>[2x]MNLKALPAIEGDHNLKNYEETYRHFDWAEAEKHFSWHETGKLNAAYEAIDRHAESFRKNKVALYYKDAKRDEKYTFKEMKEESNRAGNVLRRYGNVEKGDRVFIFMPRSPELYFIMLGAIKIGAIAGPLFEAFMEGAVKDRLENSEAKVVVTTPELLERIPVDKLPHLQHVFVVGGEAESGTNIINYDEAAKQESTRLDIEWMDKKDGFLLHYTSGSTGTPKGVLHVHEAMIQQYQTGKWVLDLKEEDIYWCTADPGWVTG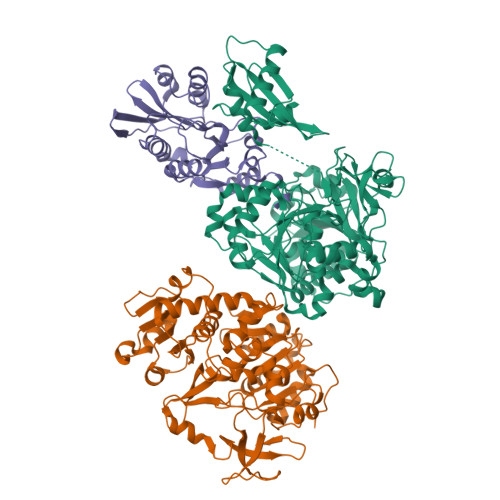TVYGIFAPWLNGATNVIVGGRFSPESWYGTIEQLGVNVWYSAPTAFRMLMGAGDEMAAKYDLTSLRHVLSVGEPLNPEVIRWGHKVFNKRIHDTWWMTETGSQLICNYPCMDIKPGSMGKPIPGVEAAIVDNQGNELPPYRMGNLAIKKGWPSMMHTIWNNPEKYESYFMPGGWYVSGDSAYMDEEGYFWFQGRVDDVIMTSGERVGPFEVESKLVEHPAIAEAGVIGKPDPVRGEIIKAFIALREGFEPSDKLKEEIRLFVKQGLAAHAAPREIEFKDKLPKTRSGKIMRRVLKAWELNLPAGDLSTMED;> MEHHKTYHSANIKTATGSLLIEGPVSPEDLAGYEFHKDLTAFRPPREQHEALVDIAGLPEGRIIIARDGRTIVGYVTYLYPDPLERWSEGNMEDLIELGAIEVAPDYRGCAVGKTLLTVSMMDEQMENYIVMTTEYYWHWDLKGMKKDVWEYRKIMEKMMNAGGLVWFATDEPEISSHPANCLMARIGKNVSQESIEQFDRLRFYHRYMY>[2x]IIDGAPCARGSHPWQVALLSGNQLHCGGVLVNERWVLTAAHCKMNEYTVHLGSDTLGDRRAQRIKASKSFRHPGYSTQTHVNDLMLVKLNSQARLSSMVKKVRLPSRCEPPG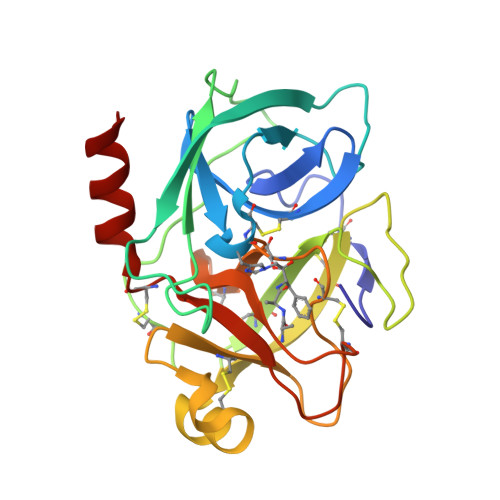TTCTVSGWGTTTSPDVTFPSDLMCVDVKLISPQDCTKVYKDLLENSMLCAGIPDSKKNACNGDSGGPLVCRGTLQGLVSWGTFPCGQPNDPGVYTQVCKFTKWINDTMKKHR>[2x]UG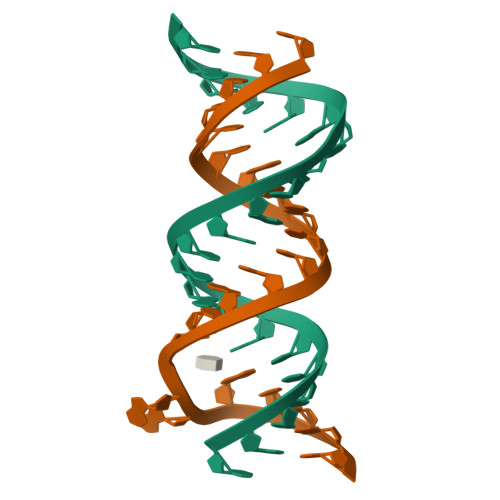CGUCACGCCGGCGAAGUCGC;>[2x]UUGCGUCACGCCGGCGAAGUCGC The INO80 complex is a universally conserved multi-subunit protein complex anchored around the Snf2 family ATPase (INO80 protein), and is involved in several DNA-related functions including chromatin remodeling, transcription regulation, replication, and DNA repair. The mammalian INO80 complex is composed of three protein modules, one of which consists of proteins specific to metazoa (animals), and not involved in ATP-dependent nucleosome remodeling. Nuclear factor related to kappa-B-binding protein (NFRKB) is a part of this module and modulates the deubiquitinase activity of UCHL5 in the INO80 complex. NFRKB enhances induced pluripotent stem cell generation and knockdown of the NFRKB gene affects the reprogramming process leading to a reduced number of human induced pluripotent stem (iPS) cell colonies.

Based on PsiPred and Disopred sequence analyses, we made 16 constructs that covered various possible boundaries of these three putative domains, and one construct, residues 370–495, produced diffraction-quality crystals. The structure of this domain was determined to 2.18 Å resolution and reveals a novel helical domain (NFRKB_WHL) bearing remarkable similarity to a winged-helix domain, usually associated with DNA binding. The crystal structure of the human NFRKB_WHL domain (residues 370–495) consists of two protomers (residues 372–483 in chain A and 370–483 in chain B), one sodium ion and 25 water molecules in the crystallographic asymmetric unit. The last 12 residues of the construct (residues 484–495) were disordered and were not modeled. The NFRKB_WHL structure adopts a fold similar to the winged-helix DNA binding fold, comprising of four α-helices, three 310-helices and a short β-sheet composed of three β-strands. Therefore, despite the structural similarity to winged-helix DNA binding domains, NFRKB_WHL is unlikely to bind DNA. The sequence of this helix lacks any basic residues, thereby making it unlikely to interact with DNA. The calculated isoelectric point of 4.3 of this domain is also not favorable for DNA binding. NFRKB_WHL has a significant structural similarity (Dali Z-score of 6.7) to one of the winged-helix motifs within the C-terminal domain (CTD) of the cullin protein portion of the of the Cul1–Rbx1–Skp1–F boxSkp2 SCF ubiquitin ligase complex. Thus, it is possible that NFRKB_WHL may be involved in protein-protein interactions rather than DNA binding.

>GLGINEISSSFFSLLLEILLLESQASLPMLEERVLDWQSSPASSLNSWFSAAPNWAELVLPALQYLAGESRAVPSSFSPFVEFKEKTQQWKLLGQSQDNEKELAALFQLWLETKDQAFCKQENEDSS[2x]> MTSSSGVDNEISLDSPMPIFNESSTLKPIRVAGVVTTGTDHIDPSVLQAYLDDTIMKSITLGQLVKNADVLNKRLCQHHIALNAKQSFHFQGNTYISDEKETHDVVPLMEVVSQLDILPPKTFTAKTGTNFGNDNDAEAYLQFEKLIDKKYLKLPTRVNLEILRGTKIHSSFLFNSYSSLSPQSILNLKVFSQFYNWNTNKGLDIGQRGARLSLRYEPLFLHKLLHNPHSNESPTLFHEWFLETCWRSTKICSQGTSAPYMYSGTMLSQAGDQLRTILGHTFVLDKRDHIMCPTKGSMLKWSNELSPGKHLKTQLELNSVKSWMNDDFITFSTTIKTGYLKNLSSQQSLPVHICDKFQSGGPSDIRGFQTFGLGPRDLYDAVGGDAFVSYGLSVFSRLPWKKVEKSNFRLHWFFNGGKLVNHDNTSLGNCIGQLSKEHSTSTGIGLVLRHPMARFELNFTLPITAHENDLIRKGFQFGLGLAFL;> MVSSFSVPMPVKRIFDTFPLQTYAAQTDKDEAVALEIQRRSYTFTERGGGSSELTVEGTYKLGVYNVFLEANTGAALATDPWCLFVQLALCQKNGLVLPTHSQEQTPSHTCNHEMLVLSRLSNPDEALPILVEGYKKRIIRSTVAISEIMRSRILDDAEQLMYYTLLDTVLYDCWITQIIFCASDAQFMELYSCQKLSGSIVTPLDVENSLLQKLSAKSLKISLTKRNKFQFRHREIVKSMQGVYHNHHNSVNQEQVLNVLFENSKQVLLGLKDMLKSDGQPTYLHLKIASYILCITNVKEPIKLKTFVENECKELVQFAQDTLKNFVQ;> MVKGSVHLWGKDGKASLISVDSIALVWFIKLCTSEEAKSMVAGLQIVFSNNTDLSSDGKLPVLILDNGTKVSGYVNIVQFLHKNICTSKYEKGTDYEEDLAIVRKKDRLLEYSLLNYVDVEISRLTDYQLFLNTKNYNEY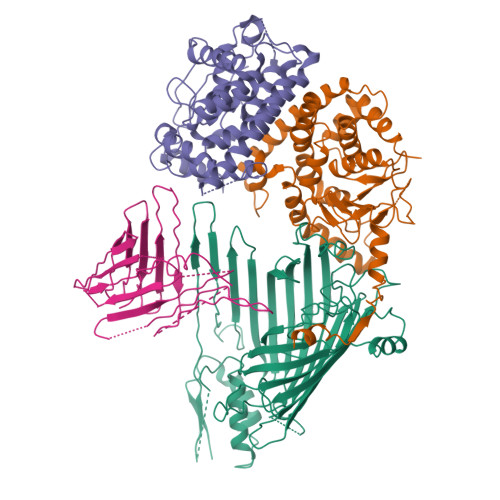TKKLFSKLLYFPMWYNTPLQLRSQARENCEEIIGSLTLEDDEEFVESKAMESASQLAQSKTFKIAHKNKIKGKQELQQVKYNLQFDNRLQSCVSNWLAARKKLDDSVILSSDLLFLANLYVQLGLPDGNRIRSKLEQTFGSELLNSMSNKIDDFVHRPSNNLEQRDPQFREQGNVVMSLYNLACKYI;> MSAPTPLAEASQIPTIPALSPLTAKQSKGNFFSSNPISSFVVDTYKQLHSHRQSLELVNPGTVENLNKEVSRDVFLSQYFFTGLRADLNKAFSMNPAFQTSHTFSIGSQALPKYAFSALFANDNLFAQGNIDNDLSVSGRLNYGWDKKNISKVNLQISDGQPTMCQLEQDYQASDFSVNVKTLNPSFSEKGEFTGVAVASFLQSVTPQLALGLETLYSRTDGSAPGDAGVSYLTRYVSKKQDWIFSGQLQANGALIASLWRKVAQNVEAGIETTLQAGMVPITDPLMGTPIGIQPTVEGSTTIGAKYEYRQSVYRGTLDSNGKVACFLERKVLPTLSVLFCGEIDHFKNDTKIGCGLQFETAGNQELLMLQQGLDADGNPLQALPQL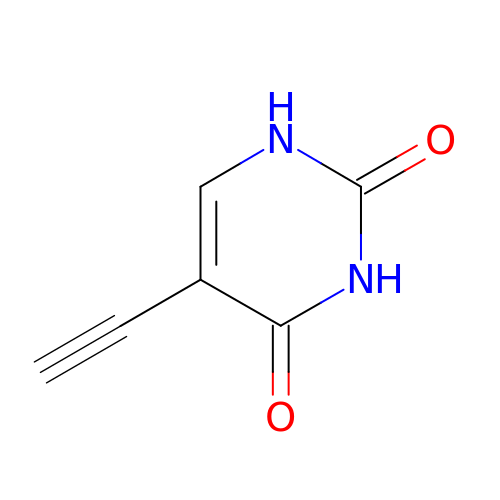5-ethynylpyrimidine-2,4(1H,3H)-dione | C6 H4 N2 O2 | JOZGNYDSEBIJDH-UHFFFAOYSA-N> MASVSPLLMPCRGVKLVNPIGKQGSQHYGLEPKLEAGRDTQLKHTEMYDGYTDDFGVFKEGPPVTLRL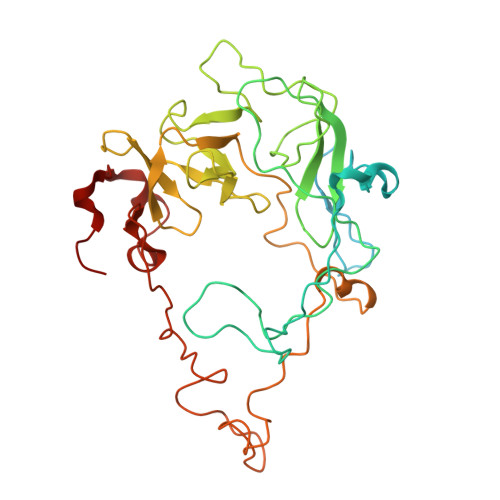EYVRSPDHGYSQHILQKDIWSPFQVGANMMSYTPLYYDWKGFSSRDYFGHRSGTNPGSKVLLGHYRRDEVRSWGYRIMVNHKPQKRIPKWLACVVHIPRKKTFLGFFLYANGAYVAELLTYKQLPRIIYNKAFQGCLPTIGQTVSLTEVTYGKEIHSVEMYPGHGGVICRASGTAAVVLRGSEPNLVPLLLPSKEVRLFDNMCHAVFGRRAGVMYNKQRNFSKRSVEENMPHRPKVHSKTKRVSSHPAGGGNGGSPNLLTPLDWRIHPRNCVKTKYWLSGYILRGRQYNRNQTVADLKSKTYSWANRDPVYR>[2x]SESLRIIFAGTPDFAARHLDALLSSGHNVVGVFTQPDRPAGRGKKLMPSPVKVLAEEKGLPVFQPVSLRPQENQQLVAELQADVMVVVAYGLILPKAVLEMPRLGCINVHGSLLPRWRGAAPIQRSLWAGDAETGVTIMQMDVGLDTGDMLYKLSCPITAEDTSGTLYDKLAELGPQGLITTLKQLADGTAKPEVQDETLVTYAEKLSKEEARIDWSLSAAQLERCI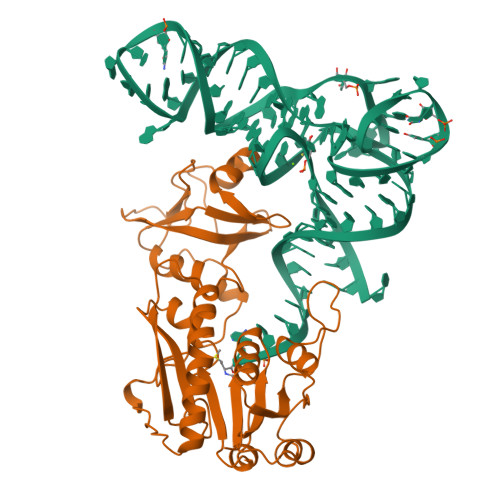RAFNPWPMSWLEIEGQPVKVWKASVIDTATNAAPGTILEANKQGIQVATGDGILNLLSLQPAGKKAMSAQDLLNSRREWFVPGNRLV> MKCLVTGGNVKVLGKAVHSLSRIGDELYLEPLEDGLSLRTVNSSRSAYACFLFAPLFFQQYQAATPGQDLLRCKILMKSFLSVFRSLAMLEKTVEKCCISLNGRSSRLVVQLHCKFGVRKTHNLSFQDCESLQAVFDPASCPHMLRAPARVLGEAVLPFSPALAEVTLGIGRGRRVILRSYHEEEADSTAKAMVTEMCL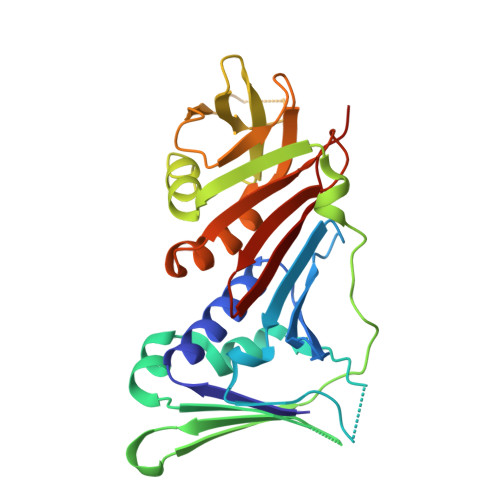GEEDFQQLQAQEGVAITFCLKEFRGLLSFAESANLNLSIHFDAPGRPAIFTIKDSLLDGHFVLATLSDTDS> SQPLIDLPLIDFCDTPEAHVAV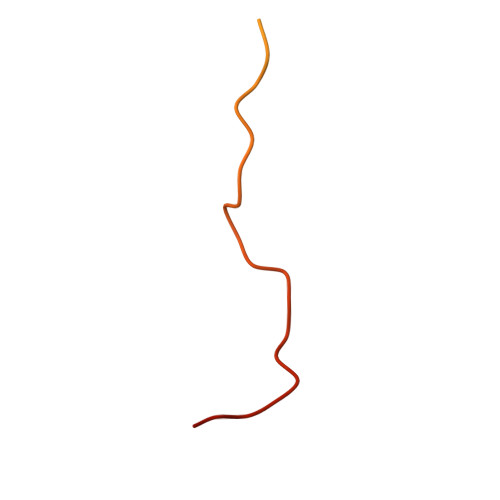GSESRPLIDLMTNTPDMNKNVAKPSPVVGQLIDLSSPLIQLSPE> MQAIKESYAFAVLGEPRYAFNFNHFDYVNPAAPKGGQITLSALGTFDNFNRYALRGNPGARTEQLYDTLFTTSDDEPGSYYPLIAESARYADDYSWVEVAINPRARFHDGSPITARDVEFTFQKFMTEGVPQFRLVYKGTTVKAIAPLTVRIELAKPGKEDMLSLFSLPVFPEKYWKDHKLSDPLATPPLASGPYRVTSWKMGQNIVYSRVKDYWAANLPVNRGRWNFDTIRYDYYLDDNVAFEAFKAGAFDLRMENDAKNWATRYTGKNFDKKYIIKDEQKNESAQDTRWLAFNIQRPVFSDRRVREAITLAFDFEWMNKALFYNAWSRTNSYFQNTEYAARNYPDAAELVLLAPMKKDLPSEVFTQIYQPPVSKGDGYDRDNLLKADKLLNEAGWVLKGQQRVNATTGQPLSFELLLPASSNSQWVLPFQHSLQRLGINMDIRKVDNSQITNRMRSRDYDMMPRVWRAMPWPSSDLQISWSSEYINSTYNAPGVQSPVIDSLINQIIAAQGNKEKLLPLGRALDRVLTWNYYMLPMWYMAEDRLAWWDKFSQPAVRPIYSLGIDTWWYDVNKAAKLPS;> LGEPRYAFNF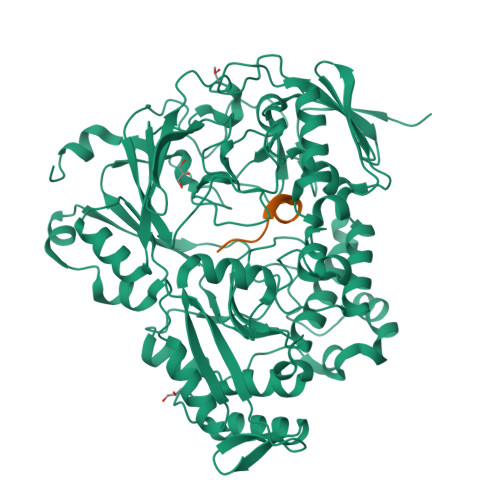N Dihydropentalenolactone F | C15 H20 O5 | 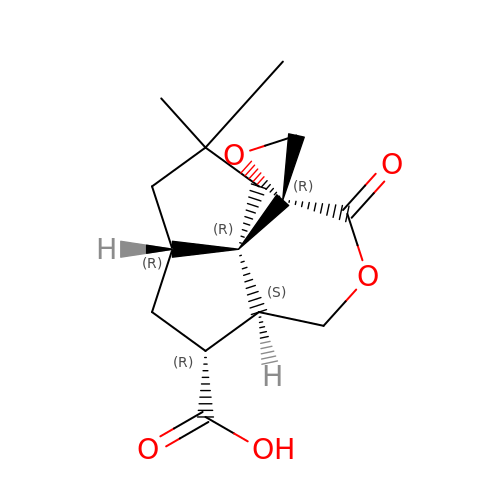FLEPJXXPLHDGAH-XKSWNSKZSA-N> TVSPYGPEARAELSSRLTTLRNTLAPATNDP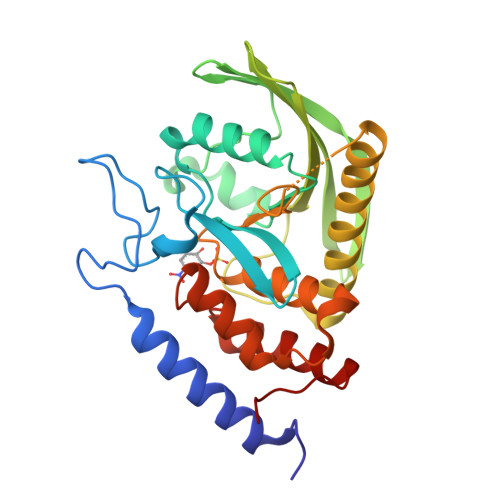RYLQACGGEKLNRFRDIQCRRQTAVRADLNANYIQVGNTRTIACQYPLQSQLESHFRMLAENRTPVLAVLASSSEIANQRFGMPDYFRQSGTYGSITVESKMTQQVGLGDGIMADMYTLTIREAGQKTISVPVVHVGNWPDQTAVSSEVTKALASLVDQTAETKRNMYESKGSSAVADDSKLRPVIHCRAGVGRTAQLIGAMCMNDSRNSQLSVEDMVSQMRVQRNGIMVQKDEQLDVLIKLAEGQGRPLLNS> MKKEVRKVRIALASPEKIRSWSYGEVEKPETI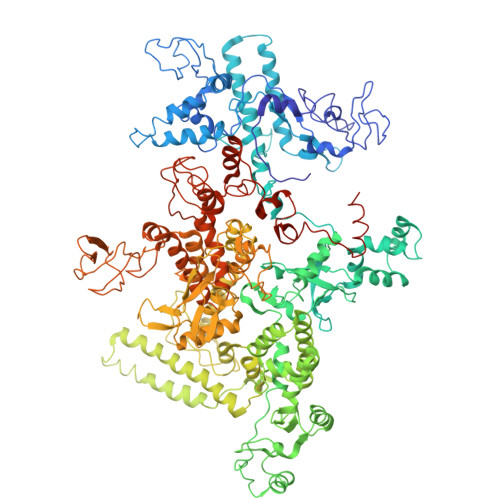NYRTLKPERDGLFDERIFGPIKDYECACGKYKRQRFEGKVCERCGVEVTRSIVRRYRMGHIELATPAAHIWFVKDVPSKIGTLLDLSATELEQVLYFNKYIVLDPKGAVLDGVPVEKRQLLTDEEYGGIDARMGAEAIQELLKELDLEKLERELLEEMKHPSRARRAKARKRLEVVRAFLDSGNRPEWMILEAVPVLPPDLRPMVQVDGGRFATSDLNDLYRRLINRNNRLKKLLAQGAPEIIIRNEKRMLQEAVDAVIDNGRRGSPVTNPGSERPLRSLTDILSGKQGRFRQNLLGKRVDYSGRSVIVVGPQLKLHQCGLPKRMALELFKPFLLKKMEEKAFAPNVKAARRMLERQRDIKDEVWDALEEVIHGKVVLLNRAPTLHRLGIQAFQPVLVEGQSIQLHPLVCEAFNADFDGDQMAVHVPLSSFAQAEARIQMLSAHNLLSPASGEPLAKPSRDIILGLYYITQVRKEKKGAGMAFATPEEALAAYERGEVALNAPIVVAGRETSVGRLKFVFANPDEALLAVAHGLLDLQDVVTVRYLGRRLETSPGRILFARIVGEAVGDEKVAQELIQMDVPQEKNSLKDLVYQAFLRLGMEKTARLLDALKYYGFTLSTTSGITIGIDDAVIPEEKQRYLEEADRKLRQIEQAYEMGFLTDRERYDQVIQLWTETTEKVTQAVFKNFEENYPFNPLYVMAQSGARGNPQQIRQLCGMRGLMQKPSGETFEVPVRSSFREGLTVLEYFISSHGARKGGADTALRTADSGYLTRKLVDVAHEIVVREADCGTTNYISVPLFQMDEVTRTLRLRKRSDIESGLYGRVLAREVEALGRRLEEGRYLSLEDVHFLIKAAEAGEVREVPVRSPLTCQTRYGVCQKCYGYDLSMARPVSIGEAVGVVAAESIGEPGTQLTMRTFHTGGVAVGTDITQGLPRVIELFEARRPKAKAVISEIDGVVRIEEGEDRLSVFVESEGFSKEYKLPKDARLLVKDGDYVEAGQPLTRGAIDPHQLLEAKGPEAVERYLVDEIQKVYRAQGVKLHDKHIEIVVRQMLKYVEVTDPGDSRLLEGQVLEKWDVEALNERLIAEGKVPVAWKPLLMGVTKSALSTKSWLSAASFQNTTHVLTEAAIAGKKDELIGLKENVILGRLIPAGTGSDFVRFTQVVDQRTLKAIEEARKEAVEAKEKEAPRRPVRREQPGKGL>SNAMDSRFLPATAFIDPEGRNRNEVERLVQQVVDLILAKLTGAAERPPMPETVDLPGPITIPEAAATEATLLQAIRDMVDGSMNPANPGYIGHMDPMPATMAILGDLVAAAVNNNMLSLEMSPSFSRLETLLLRAIAGLFGLGEQAGGVLTSGGSLANLQALAVARNVAFDSVEPGITGLAQRPVIFASEAAHTSLQKAAMLLGLGTAAVIPVRATADSRMDPEDLRARIDQARGAGQHPFCVVATAGTTTTGNIDPLAEIGAIAREHGLWFHVDAAYGGALVFSERHRWRLAGIEQADSITFNPQKWLYVAKTCAMVLFRDAGVLERAFRIPAPQMRATDGFINLGEIGVQGTRHADVVKLWLTLQHIGQ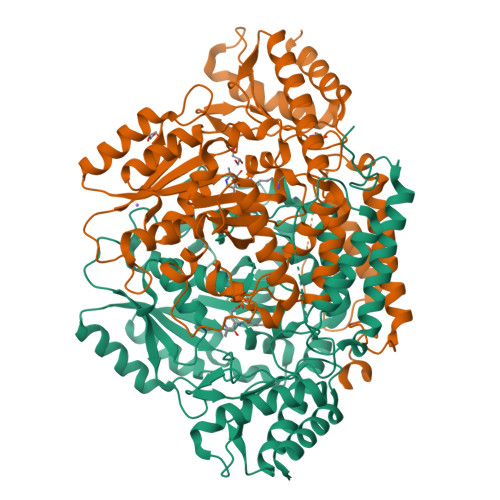QGYARLIDDGYRLAERVVEGVRQRPFLRLAGEIDTNIVCFRGEPDWLPAERWDDWNAALQALLLREGKIFLSLPVYRGGRWLRAVLLNPYTTDAVIDAMFKQIDRFAGRERGQER[4x]L-gamma-glutamyl-S-[(2-phenylethyl)carbamothioyl]-L-cysteinylglycine | C19 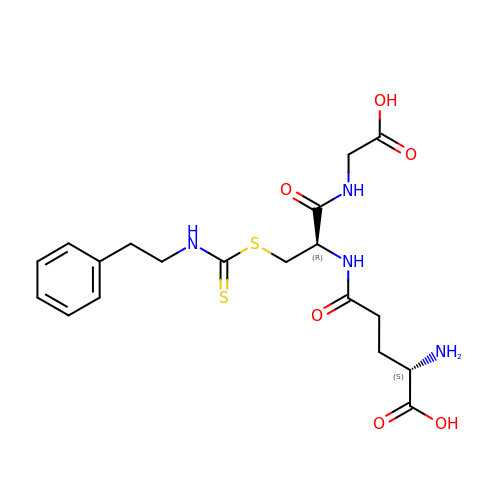H26 N4 O6 S2 | WSGBVCNCZSZCGE-KBPBESRZSA-N> MLSPEALTTAVDAAQQAIALADTLDVLARVKTEHLGDRSPLALARQALAVLPKEQRAEAGKRVNAARNAAQRSYDERLATLRAERDAAVLVAEGIDVTLPSTRVPAGARHPIIMLAEHVADTFIAMGWELAEGPEVETEQFNFDALNFPADHPARGEQDTFYIAPEDSRQLLRTHTSPVQIRTLLARELPVYIISIGRTFRTDELDATHTPIFHQVEGLAVDRGLSMAHLRGTLDAFARAEFGPSARTRIRPHFFPFTEPSAEVD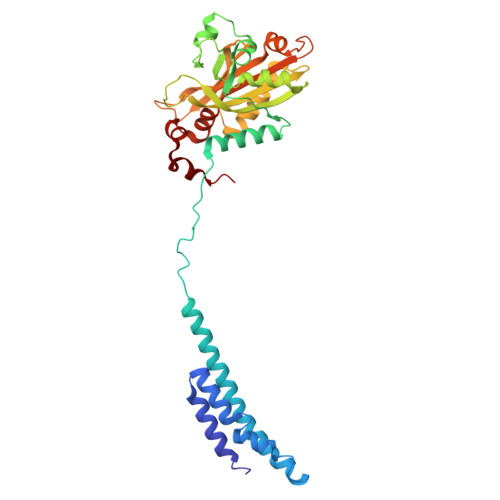VWFANKIGGAAWVEWGGCGMVHPNVLRATGIDPDLYSGFAFGMGLERTLQFRNGIPDMRDMVEGDVRFSLPFGVGA>TRKAVIGYYFIPTNQINNYTETDTSVVPFPVSNITPAKAKQLTHINFSFLDINSNLECAWDPATNDAKARDVVNRLTALKAHNPSLRIMFSIGGWYYSNDLGVSHANYVNAVKTPASRAKFAQSCVRIMKDYGFDGVDIDWEYPQAAEVDGFIAALQEIRTLLNQQTITDGRQALPYQLTIAGAGGAFFLSRYYSKLAQIVAPLDYINLMTYDLAGPWEKVTNHQAALFGDAAGPTFYNALREANLGWSWEELTRAFPSPFSLTVDAAVQQHLMMEGVPSAKIVMGVPFYGRAFKGVSGGNGGQYSSHSTPGEDPYPSTDYWLVGCEECVRDKDPRIASYRQLEQMLQGNYGYQRLWNDKTKTPYLYHAQNGLFVTYDDAESFKYKAKYIKQQQLGGVMFWHLGQDNRNGDLLAALDRYFNAADYDDSQLDMG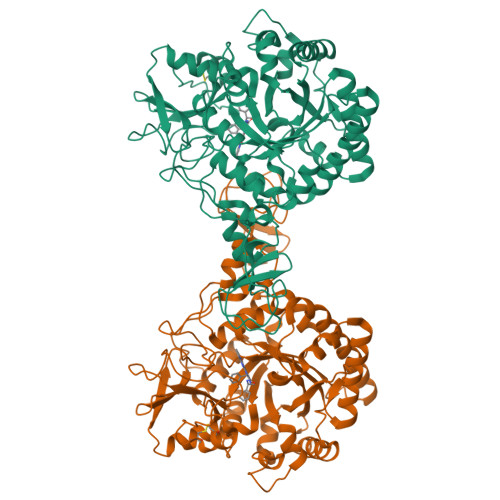TGLRYTGVGPGNLPIMTAPAYVPGTTYAQGALVSYQGYVWQTKWGYITSAPGSDSAWLKVGRV[2x]>[2x]LYFPQRLYTENIYVGQQQGSPLLQVISMREFPTERPYFFLCSHRDAFTSWFHIDEASGVLYLNKTLEWSDFSSLRSGSVRSPKDLTLKVGVSSTPPMKVMCTILPTVEVKLSFINDTAPSCGQVELSTLCFPEKISNPHITENREPGALRQLRRFTHMSICPNYTISYGVVAGSSVPFAVDDSTSELVVTAQVDREEKEVYHLDIVCMVRTERNLEEVFRSLHVNIYDEDDNSPYVQGTD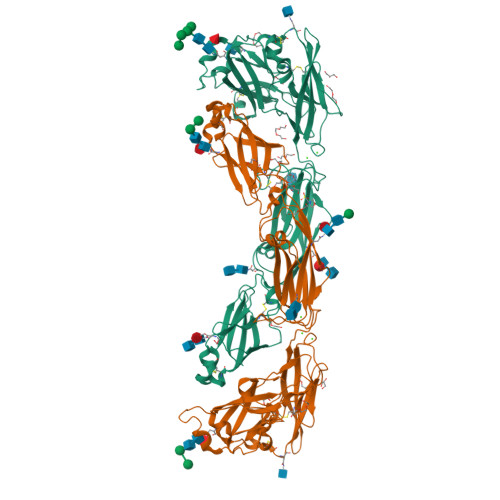TEDVLVEFDRSEGTVFGTLFVYDRDTTPVYPTNQVQNKLVGTLMTQDSWIKNNFAIEHKFREEKAIFGNVRGTVHEYKLKLSQNLSVTEQRSFLLGYLVNDTTFPGPEGTVLLHFNVTVLPVPIRFSQVTYSFTVSQKATTYSQIGKVCVENCQKFKGIDVTYQLEIVDRQITAEAQSCYWAVSLAQNPNDNTGVLYVNDTKVLRRPECQELEYVVIAQEQQNKLQAKTQLTVSFQGEAD>KLCLVCSDEASGCHYGVL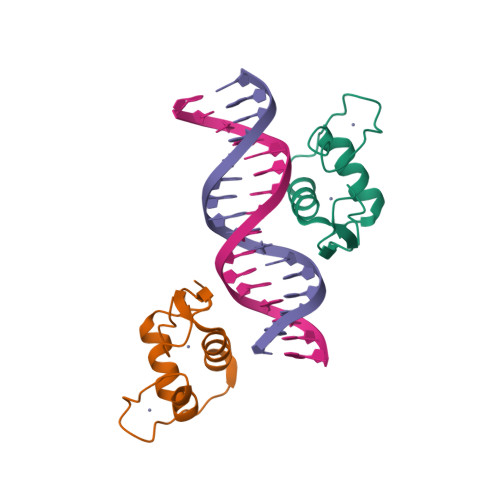TCGSCKVFFKRAVEGQHNYLCAGRNDCIIDKIRRKNCPACRYRKCLQAGMNLEA[2x]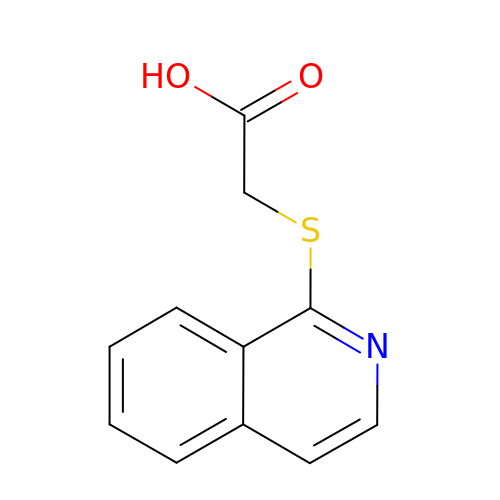2-isoquinolin-1-ylsulfanylethanoic acid | C11 H9 N O2 S | PISYQRRSPUEVQL-UHFFFAOYSA-N> MGSSHHHHHHSSGRENLYFQGMIKEMIEDFISKGGLIFTHSGRYTNTNNSCFIFNKNDIGVDTKVDMYTPKSAGIKNEEGENLWQVLNKANMFYRI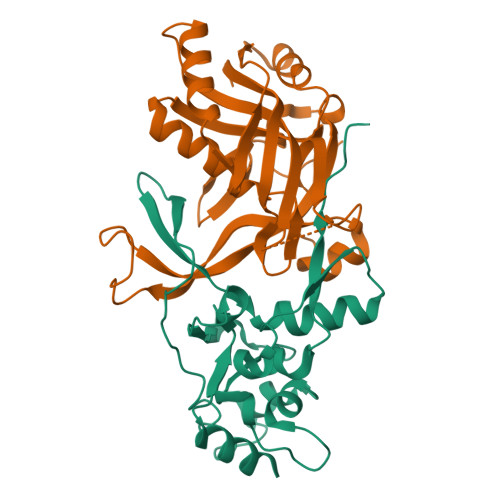YSGELGEELQYLLKSCCTAKEDVTTLPQIYFKNGEGYDILVPIGNAHNLISGTEYLWEHKYYNTFTQKLGGSNPQNCTHACNKMRGGFKQFNCTPPQVEDNYNA;> MGSSHHHHHHSSGRENLYFQGMRKFIIVKNVKVDGINAKSSDITVGMPPATTFCGLGETMSIKTGIVVKAVSYGSVKFEVRGSRFNTSVTKFAWQDRGNGGKANNNSPIQPKPLADGVFTLCFEVEWEDCAEVLVDKVTNFINTARIAGGTIASFNKPFVKVAKDAEELASVKNAMMPCYVVVDCGVEVNIFEDAVNRKLQPMVNGYKKLEKIVDNKHMRDKFTPAYLATPTYTMIGYKMVSNVDNFDQALWQYGENTKVKTIGGIYND>GPGSSHWTSKVHESVIGRNPEGQLGFELKGGAENGQFPYLGEVKPGKVAYESGSKLVSEELLLEVNETPVAGLTIRDVLAVIKHCKDPLRLKCVKQGGIVDKDLRHYLNLRFQKGSVDHELQQIIRD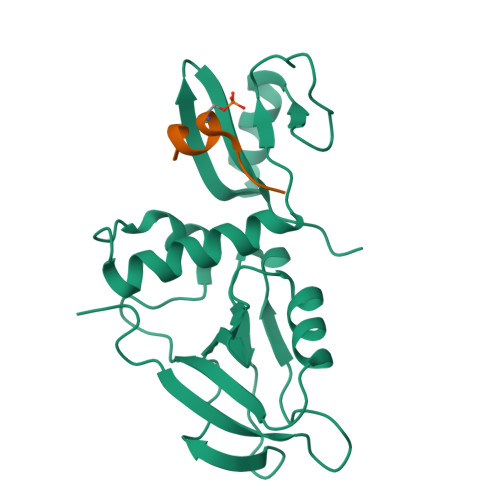NLYLRTVPCTTRPHKEGEVPGVDYIFITVEEFMELEKSGALLESGTYEDNYYGTPKPPAEPAPLLNVTDQILPGATPSAEGKRKRNKSVTNMEKASIEPPEEEEEER[2x];>NLRNQSYRAAMK[2x]>GAH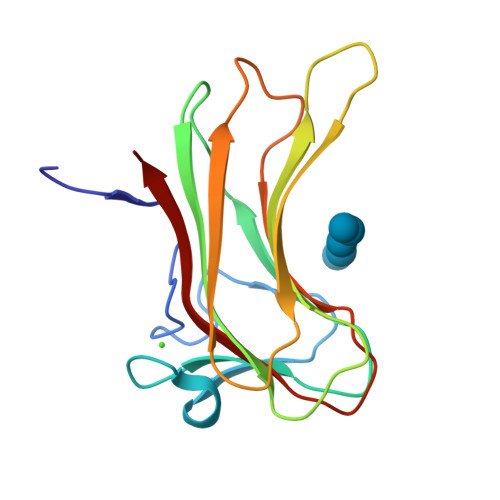MVNMVSNPGFEDGLDSWQDWQQDMSAVPEAAHNGALGLKIGGGKAAGGGQDIPLKPNTTYILGAWAKFDSKPAGTFDVVVQYHLKDANNTYVQHILNFNETDWTYKQLLFTTPDVFGSTPQLALWKGDTSKANLYVDDVYLVEV[2x]> GH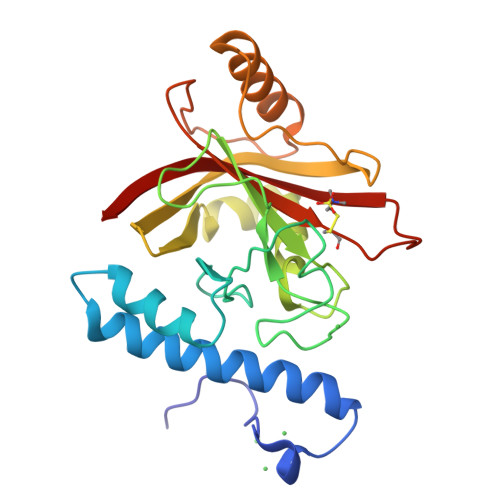HHHHHHHHHSSGHISGDAMEDKQERANYEKLQQKFQMLMSKHQAHVRPQFESLEKINKDIVGWIKLSGTSLNYPVLQGKTNHDYLNLDFEREHRRKGSIFMDFRNELKNLNHNTILYGHHVGDNTMFDVLEDYLKQSFYEKHKIIEFDNKYGKYQLQVFSAYKTTTKDNYIRTDFENDQDYQQFLDETKRKSVINSDVNVTVKDRIMTLSTCEDAYSETTKRIVVVAKIIKVS>[2x]SRAPAPATPHAPDHSPAPNSPTLTRPPEGPKFPRVKNWELGSITYDTLCAQSQQDGPCTPRRCLGSLMLPRKLQTRPSPGPPPAEQLLSQARDFINQYYSSIKRSGSQAHEERLQEVEAEVASTGTYHLRESELVFGAKQAWRNAPRCVGRIQWGKLQVFDARDCSSAQEMFTYICNHIKYATNR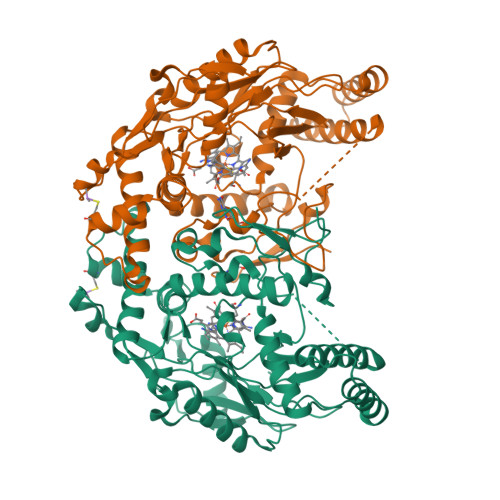GNLRSAITVFPQRAPGRGDFRIWNSQLVRYAGYRQQDGSVRGDPANVEITELCIQHGWTPGNGRFDVLPLLLQAPDEAPELFVLPPELVLEVPLEHPTLEWFAALGLRWYALPAVSNMLLEIGGLEFSAAPFSGWYMSTEIGTRDLCDPHRYNILEDVAVCMDLDTRTTSSLWKDKAAVEINLAVLHSFQLAKVTIVDHHAATVSFMKHLDNEQKARGGCPADWAWIVPPISGSLTPVFHQEMVNYILSPAFRYQPDPW> MFHFIPSWYNENRTWYDNNYLWYFKPTNVGFDDTINQMKMFDYAGKESRLVVLNYMPNLRYYLHRYDLLESGYYSVFDDIQEIGNVRQQMIDFRQLNWPEGVDFTYTPFIVLVKKSGDLIAKVQFGEEGNLTHIDYFANEQIAKKYLFDDRGFLSSILYYDNGGEAYQDYLAPSGERIMREYLREGDHHVEINPKKAIHFLKLSYSDIEELIREKYLTYLHKEVSKSDTIIVSFNQVHNAFIVGNTSKGNLILSVFSERNNAHNVLEDYSSLSRADAIICDRLDIAAQLKEKIDKPVVHVSPFDTRLALGKSNQVRDLEIYFVVDRLSHKELQKSLTSLYKVMLKNNDIKVTFVSYEREFESRQLTYDYLKEATKVFDQKFFSLSDDDANQVLMQSDEVEKEKTRLSFTHPLSETDIINRLEYVRLIIDISKIPDLYTQIAGISSGIPQINTILTEFVEHRKNGYIIEEIQELEKAIPYYCEQLTNWNRSLIYSIDKINDYTGGQLVERIINSY;> MSKIKLTILQVGEENWATKENIPNNMEWLFIKPDQISDFVTTENNYLTSSKLLQKLPRKISALLLTEQTYGPELSSLSSFFEVYEVFYPKDKHATGITEEFLRSKMAQRYDSSSPDQLIRQFYKGLFIGQYGEKLQVSQIQIRNDFEGVVNYQGNNYLELEGQFGENYSFLLNFAYNIPFSSDFYNELFLEHIIEGDIDIRLVISLIVDGSVDDIAKEWYFEKEDLNQLISLESDISGSLAVKLFAKGKGIVKLGPLHRRNGRGGLGTFLLGGERHIDAIGHEFMTYFDPVDFKPPLTVYFSGFRSAEGFEGFWMMKSMKTPFMLICDPRLQGGAFYIGSKEYEQKIVDAIQEKLAFLNFSSDQLILSGLSMGTYGATYHGAKLNPHAIIIGKPIFNLGTVAQRERLERPDGFATSL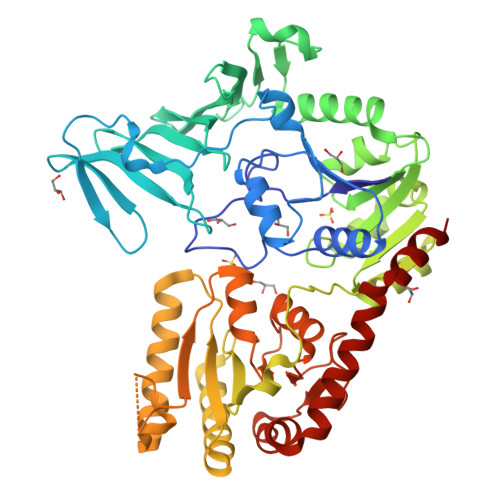DIQLLNQGDLTSSSSEKLNNYFWKSIEEGDFSNTTFALAYMKNDDYDATAFSDLLQYFRGKKHKILGRGWDGRHGDCSAEVGAWFTSQYRRMLSNDFGRKEE;> MSTISYIYWDDFSRFSYNFGTKLQFLGKSVCFENPLAPSSTNLYTWSSQTNYQSKRISPNLPLLRKGTRYSLSLNAELDLVSSLFVRIEFYNRFNESVGFELLKKDSIIFIYPKEAYTYTISLINAGCSDFTFHYLKLEEVTDSVIQEKNLSTEFTIEEHQDVLNLLLVEKKDSVYINKIESISQLQQKVELVSNPSLNSDSLILPELEKGLEDALKVFPNIKINVIAYGTQGNFAALYYAKKFPRITAYINDCFAPFGILLKSLPHLTAKQQIFLREVWDTRETSPNVKHYGLVSENSSLNLVSMILSGNEHLPYLTLLKKQDDNYDSL>GMNNIAYIALGSNIGERYTYLTEAIQFLNKNPYIKVEDVSS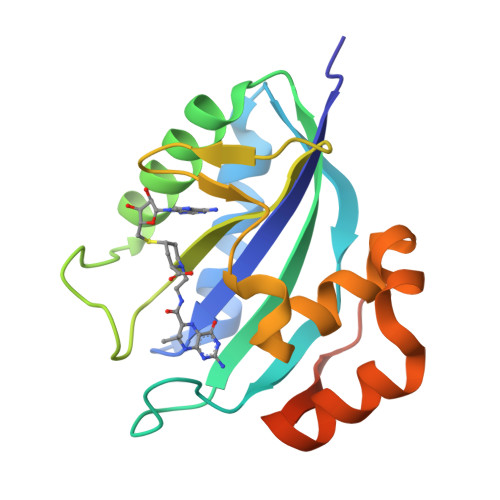VYETEPVGYTDQSCFLNLVIKISTNLSPQELLKVTQKVENDLGRKREIRWGPRTIDLDILLYNQENIEAENLIVPHPRMFERAFVIVPLLEINQDIKQNISRSQVEEMKRREGVTVWKQKNGEDAFVLFEN[2x]>MVESNDIIKSGLAEKALKALILQCEENPSLKNDKDIHIIINTGKKMGINRDNIPRIIPLTKYKLFKPRDLNI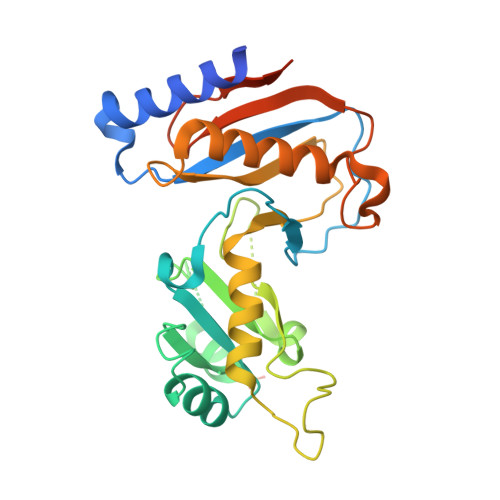LLITKDPSALYRETLTKDEHTSELFKEIISVKNLRRRFKGSKLTQLYKDFDLVVADYRVHHLLPEVLGSRFYHGSKKLPYMIRMSKEVKLKRQQMVEKCDPIYVRAQLRSICKNTSYIPNNDNCLSVRVGYIQKHSIPEILQNIQDTINFLTDKSKRPQGGVIKGGIISIFVKTSNSTSLPIYQFSEARENQKNEDLSDIKL[2x]~{N}-[5-methyl-4-[7-[[(2~{R})-2-(4-methylpiperazin-1-yl)propanoyl]amino]-1~{H}-indol-3-yl]pyrimidin-2-yl]cyclopropanecarboxamide 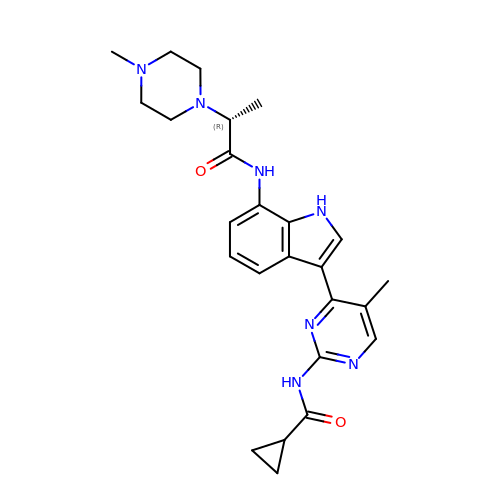| C25 H31 N7 O2 | IMKONRLYDLGQAV-MRXNPFEDSA-N>XXXXXXXXXXXXXXPSNPNSPSAQLAKEEQRRKKRRLKKRIFAAVSEGCVEELVELLVELQELCRRRHDEDVPDFLMHKLTASDTGATCLMKALLNINPNTKEIVRILLAFAEENDILGRFINAEYTEEAYEGQTALNIAIERRQGDIAALLIAAGADVNAHAKGAFFNPKYQHEGFYFGETPLALAACTNQPEIVQLLMEHEQTDITSRDSRGNNILHALVTVAEDFKTQNDFVKRMYDMILLRSGNWELETTRNNDGLTPLQLAAKMGKAEILKYILSREIKEKRLRSLSRKFTDWAYGPVSSSLYDLTNVDTTTDNSVLEITVYNTNIDNRHEMLTLEPLHTLLHMKWKKFAKHMFFLSFCFYFFYNITLTLVSYYRPREEEAIPHPLALTHKMGWLQLLGRMFVLIWAMCISVKEGIAIFLLRPSDLQSILSDAWFHFVFFIQAVLVILSVFLYLFAYKEYLACLVLAMALGWANMLYYTRGFQSMGMYSVMIQKVILHDVLKFLFVYIVFLLGFGVALASLIEKCPKDNKDCSSYGSFSDAVLELFKLTIGLGDLNIQQNSKYPILFLFLLITYVILTFVLLLNMLIALMGETVENVSKESERIWRLQRARTILEFEKMLPEWLRSRFRMGELCKVAEDDFRLCLRINEVKWTEWKTHVSFLNEDPGPVRRTDFNKIQDSSRNNSKTTLNAFEEVEEFPETSVVDAGLEVLFQGDYKDDDDKAHHHHHH[4x]

The Transient Receptor Potential Vanilloid (TRPV) channel subfamily is a subset of the large TRP channel superfamily, and consist of subtypes TRPV1-TRPV6. TRPV1-4 are intrinsically temperature sensitive (thermoTRPV) and have been found to play important roles in numerous physiological processes including thermosensation, nociception, and osmosensation. TRPV3 exhibits use-dependent increase in current amplitudes (termed sensitization) upon repeated applications of either ligand or heat. The combination of our structural data and functional experiments provides evidence that hysteresis, sensitization, and activation of TRPV3 involves increased coupling between structural elements from the cytoplasmic (ARD and CD) and the transmembrane domains (TRP and S6) is triggered by a coil-to-helix transition in the distal CTD.

In order to elucidate the conformational changes that underlie the transition to the sensitized C1 state, we introduced the K169A mutation into the hTRPV3 carrying the previously reported functionally silent T96A mutation (TRPV3K169A in future references). We expressed and purified the TRPV3K169A channel and solved its structure by single particle 3D cryo-electron microscopy (cryo-EM) (Figure 2—figure supplements 1 and 2). By contrast, the K169A mutation induces a substantial change in the secondary structure and the position of the distal CTD as well as the ARD-CTD interface. Specifically, the distal CTD undergoes a dramatic coil-to-helix transition and this newly formed helical distal CTD is positioned behind the βCD in the cytoplasmic vestibule of the channel. Furthermore, the cryo-EM map of the TRPV3K169A contains a protein density that abuts the proximal CTD and the CD and occupies a similar space to that vacated by the distal CTD upon coil-to-helix transition. Instead, the density appears to be connected to the N-terminal of the neighboring protomer to which connectivity is visible at low contours of the map. Since this density is not sufficiently resolved to allow for unambiguous model building, we built this putative N-terminal region as a polyalanine chain. The coil-to-helix transition in the distal CTD and the rearrangement of the putative N-terminal region in the TRPV3K169A are accompanied by an apparent anti-clockwise rotation of the ARD when viewed from the extracellular space. Notably, while the distal CTD of TRPV3K169A does not contribute to the front side of the interface with minimal interaction with the CD of its own protomer, it forms extensive interactions with the loop of AR5 of the neighboring subunit at the back side of the interface.>SDQIVREHYNERTIIANRAKRNLSPIIKLRNFNNAIKYMLIDKYTKPGDVVLELGCGKGGDLRKYGAAGISQFIGIDISNASIQEAHKRYRSMRNLDYQVVLITGDCFGESLGVAVEPFPDCRFPCDIVSTQFCLHYAFETEEKARRALLNVAKSLKIGGHFFGTIPDSEFIRYKLNKFPKEVEKPSWGNSIYKVTFENNSYQKNDYEFTSPYGQMYTYWLEDAIDNVPEYVVPFETLRSLADEYGLELVSQMPFNKFFVQEIPKWIERFSPKMREGLQRSDGRYGVEGDEKEAASYFYTMFAFRKVKQYIEPESVKPN[2x]

The essential enzyme messenger RNA (mRNA) (guanine-N7) methyltransferase catalyzes S-adenosylmethionine (SAM)-dependent conversion of GpppRNA ends to the m7GpppRNA cap structure characteristic of eukaryal mRNAs. The antibiotic sinefungin (SFG) is a SAM analog in which the S-CH3 sulfonium moiety of SAM is replaced by a C-NH2 amine. Available evidence indicates that the antifungal activity of SFG is exerted via inhibition of fungal cap methyltransferase Abd1. Crystal structures of K. lactis and S. cerevisiae Abd1 as binary complexes with SAH or SFG and ternary complexes with GTP•SFG highlight how SFG makes two hydrogen bonds from its C-NH2 amine to the guanine-O6 and -N7 atoms of GTP that account for its higher affinity vis-à-vis SAH and SAM.

We co-crystallized a ScAbd1Δ119•SFG•GTP ternary complex by preincubating the protein with 0.7 mM SFG and 1 mM GTP. The structure was refined at 1.45 Å resolution with Rwork/Rfree of 12.7/15.2. The crystal contained two protomers in the asymmetric unit. Electron densities corresponding to SFG and GTP were observed in the methyl donor and acceptor sites, respectively. No interpretable electron density was seen for the N-terminal segment of either protomer (aa 120–140). In the methyl donor site of ScAbd1, SFG interacts with a similar ensemble of conserved residues as seen in KlAbd1. In the ScAbd1•SFG•GTP ternary complex, the C-NH2 amine of SFG makes hydrogen bonds to the guanine-O6 (3.0 Å) and -N7 (2.8 Å) atoms of GTP and also to the backbone carbonyl of Phe250 (2.8 Å). The GTP guanosine in the ScAbd1 methyl acceptor site interacts with a set of conserved residues analogous to the contacts observed in the KlAbd1•SFG•GTP ternary complex. The electron density maps highlighted two alternate conformations for the triphosphate moiety of GTP, entailing different direct and water-mediated contact with surrounding positively charged side chains and the SFG amine and carboxylate groups. The conformational heterogeneity of the GTP may stem from the fact that it lacks the 5′ nucleotides of GpppRNA, the physiological substrate for Abd1.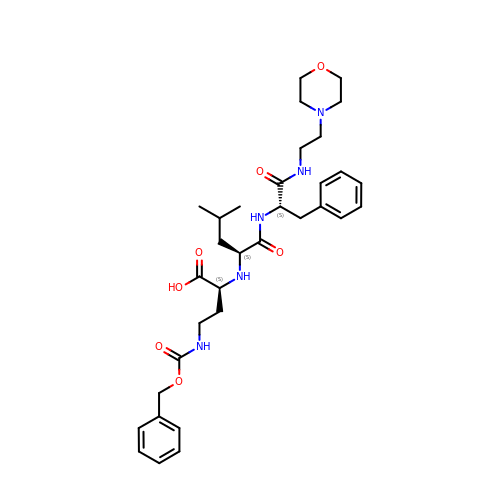N-[(1S)-3-{[(benzyloxy)carbonyl]amino}-1-carboxypropyl]-L-leucyl-N-(2-morpholin-4-ylethyl)-L-phenylalaninamide | C33 H47 N5 O7 | XQSMAYNMHYYWCR-ULNSLHSMSA-N>[3x]GSHMEWYFGKLGRKDAERQLLSFGNPRGTFLIRESETTKGAYSL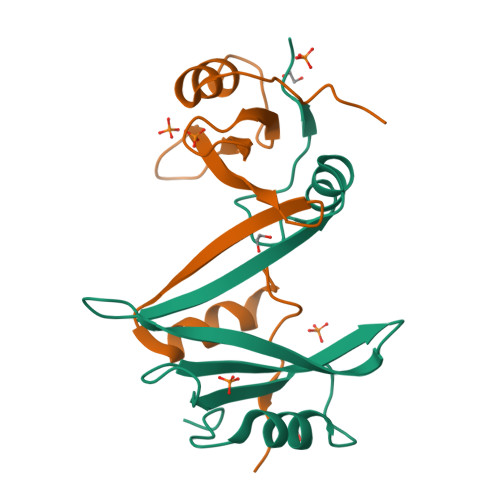SIRDWDDMKGDHVKHYKIRKLDNGGYYITTRAQFETLQQLVQHYSERAAGLCCRLVVPCHK>MAHHHHHHSSGLEVLFQGPADTLQSLAILGATGSIGDSTLAIIRQHPNRYRIHALTGFSRVDKLLALAMEFHPVKICTSPDNYAQLSQKVTDAGLDTIILSGDEGLIEIASDEAVDTVVAAIVGAAGLSSTLAAAGAGKRILLANKESLVMAGDLVIKTAKKHGATILPIDSEHNAIYQCLPAAIQADNTAIHHTSYGIKKLWLTASGGSFLDKSIKQMQNASVKEAVNHPNWSMGQKISIDSATMMNKGLELIEACHLFDLKEHQIQVVIHPNSVVHSLVEYVDGSFLAQLGTPDMKTPIAHALAYPERIKSGVMPLDLYQLGSLKFLAPDLDKFAC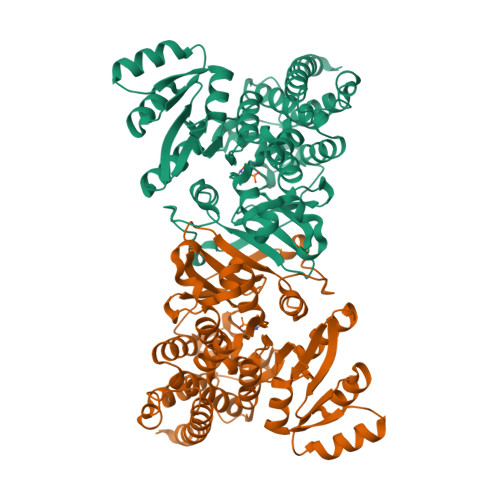LKLARYAARLGTGACIALNTANEIAVEAFLAEKICLTDIAVIVKACLDDKTIAQDYSQDFGDEVLGLERILTMDKKVRKIATAKIKLLKQGDVL[2x]>[2x]GTNRQTERIKRQREAVPLTEVGSQCRLTFKLPGISPFDLGATVTSPGGVTEAAEIGEVEDGLYGVNFVP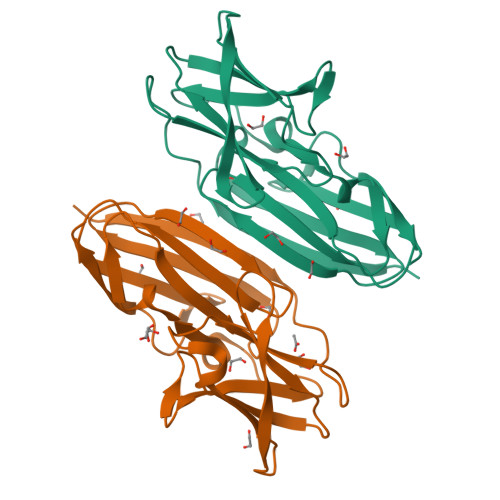KELGVHTVSVKYQEMHIPGSPFQFTVGPLKDGGAHRVHAGGPGLERGEQGMPNEFNVWTREAGAGSLAISVEGPSKAEIDFKDRKDGSCYVSYVVAEPGEYRVGIKFNDKHIPDSPYKVYITPSLGE>GAMGMKEKEESIQLHQEAWERHHLRKELRSKNQNAPDSRPEENFFSRLDSSIKKNTAFVKKLKTITEQQRDSLSHDFNGLNLSKYIAEAVASIVEAKLKISDVNCAVHLCSLFHQRYADFAPSLLQVWKKHFEARKEEKTPNITKLRTDLRFIAELTIVGIFTDKEGLSLIYEQLKNIINADRESHTHVSVVISFCRHCGDDIAGLVPRKVKSAAEKFNLSFPPSEIISPEKQQPFQNLLKEYFTSLTKHLKRDHRELQNTERQNRRILHSKGELSEDRHKQYEEFAMSYQKLLANSQSLADLLDENMPDLPQDKPTPEEHGPGIDIFTPGKPGEYDLEGGIWEDEDARNFYENLIDLKAFVPAILFKDN[2x]

Nonsense-mediated mRNA decay (NMD) is a eukaryotic mRNA quality control mechanism that recognizes transcripts with premature termination codons (PTC) and promotes their degradation. Human UPF2 (Q9HAU5) is an ∼140 kDa protein containing three conserved MIF4G (Middle portion of eIF4G) domains that are found in a number of proteins involved in RNA metabolism and translation such as the nuclear cap-binding protein CBP80 and eIF4G (eukaryotic initiation factor 4-gamma). UPF2 interacts via its third MIF4G domain with UPF3b and via its C-terminal extremity with UPF1, thus forming the central component of the ternary complex of UPF proteins. Here, we present the atomic resolution crystal structures of the N-terminal (MIF4G-1) and middle (MIF4G-2) domains of UPF2 and a lower resolution crystal structure of the combined UPF2 MIF4G-2/MIF4G-3 domains.

MIF4G-1 helices hA, hB as well as their adjacent loops make extensive contacts with the 10-helix MIF4G core domain, in particular with helices h4, h6 and h8. Notably, Arg137 and Arg141 on hA form hydrogen bonds and salt bridges with Asp317 and Glu271 on the core MIF4G domain, and Leu144 on hA interacts with Val223 and Val275 on h4 and h6, respectively. Pro156, Phe160, Phe161 and Leu164 on hB form a hydrophobic patch interacting with Arg232 and Tyr233 on helix h4. Overall, helices hA, hB and h8i create an extensive network of interactions with the 10 conserved helices of MIF4G-1 core MIF4G domain. A highly conserved motif, 164-LDSSLKKNT-172, is located on the first turn of h1 and the loop immediately preceding it. Mapping of phylogenetically conserved residues on the solvent-accessible surface of MIF4G-1 shows that the motif and a series of downstream conserved charged residues (Lys176, Lys177, Lys179, Asp192, Lys200, Glu204 and Glu211) define a conserved patch at one extremity of the domain. Residues 430–486 at the C-terminus of the MIF4G-1 crystallization construct are disordered in the crystal structure. In addition to the N-terminal extension, MIF4G-1 contains two elongated helices (h9 and h10). The updated quasi-atomic model indicates that (i) the long coiled coil formed by helices h9 and h10 protruding from MIF4G-1 is in close proximity to and could contact the EJC, (ii) the loop between h9 and h10 contacts MIF4G-2 and (iii) the MIF4G-2 domain is positioned close to the Y14 subunit of the EJC likely forming a contact.>LKCYQHGKVVTCHRDMKFCYHNTGMPFRNLKL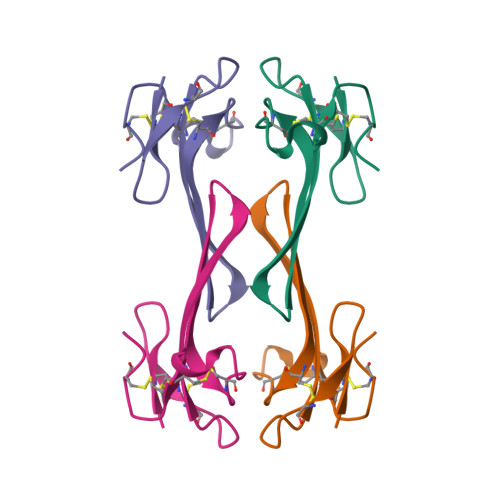ILQGCSSSCSETENNKCCSTDRCNK[2x]3-acetyl-1-((3-(1-cyclopropyl-1H-pyrazol-4-yl)-2-fluoro-5-(hydroxymethyl)phenyl)carbamoyl)indolizin-7-yl dimethylcarbamate | C27 H26 F N5 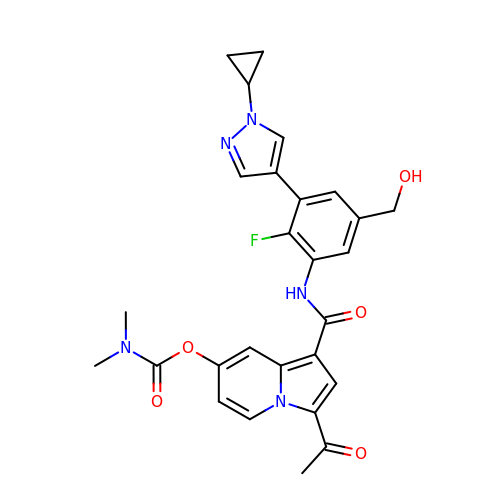O5 | UMURGYUDULFAPH-UHFFFAOYSA-N>[2x]GPLGSMELKYNCILNIKYEMDRDKLVDSSGYRSRINIGTGVKFSEIDKNQVQLSNLESSKIEVILNN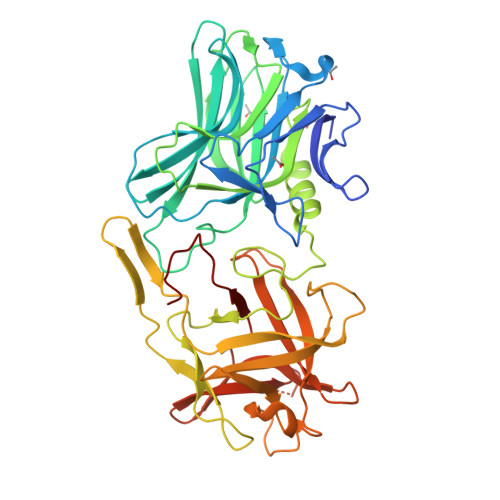GVIYNSMYENFSTSFWIRIPKYFRNINNEYKIISCMQNNSGWEVSLNFSNMNSKIIWTLQDTEGIKKTVVFQYTQNINISDYINRWIFVTITNNRLSNSKIYINGRLINEESISDLGNIHASNNIMFKLDGCRDPHRYIWIKYFNLFDKELNKKEIKDLYDNQSNSGILKDFWGDYLQYDKPYYMLNLYDPNKYLDVNNVGIRGYMYLKGPRGRIVTTNIYLNSTLYMGTKFIIKKYASGNKDNIVRNNDRVYINVVVKNKEYRLATNASQAGVEKILSAVEIPDVGNLSQVVVMKSENDQGIRNKCKMNLQDNNGNDIGFIGFHQFNNIAKLVASNWYNRQIGKASRTFGCSWEFIPVDDGWGESSL>[2x]ADPGTSECSVIGYNAICINRGLHQVPELPAHVNYVDLSLNSIAELNETSFSRLQDLQFLKVEQQTPGLVIRNNTFRGLSSLIILKLDYNQFLQLETGAFNGLANLEVLTLTQCNLDGAVLSGNFFKPLTSLEMLVLRDNNIKKIQPASFFLNMRRFHVLDLTFNKVKSICEEDLLNFQGKHFTLLRLSSITLQDMNEYWLGWEKCGNPFKNTSITTLDLSGNGFKESMAKRFFDAIAGTKIQSLILSNSYNMGSSFGHTNFKDPDNFTFKGLEASGVKTCDLSKSKIFALLKSVFSHFTDLEQLTLAQNEINKIDDNAFWGLTHLLKLNLSQNFLGSIDSRMFENLDKLEVLDLSYNHIRALGDQSFLGLPNLKELALDTNQLKSVPDGIFDRLTSLQKIWLHTNPWDCSCPRIDYLSRWLNKNSQKEQGSAKCSGSGKPVRSIICPTSASLVPR;>GSAKDPGQIRGLEMASKNSQDGISLIQTAEGALTETHAILQRMRELTVQAGNTGTQQAEDLGAIKDEMDALIEEIDGISNRTEFNGKKLLDGTNSTDGFTFQIGANAGQQLNVKIDSMSSTALGVNALDVTDFAATAFDDQLKSIDTAINTVSTQRAKLGAVQNRLEHTINNLGASGENLTAA[2x]

Flagellin is a structural protein that assembles into the lash-like filament of a bacterial flagellum, which extends from the cell surface and allows bacteria to be motile. Upon bacterial invasion, flagellin is detected by Toll-like receptor 5 (TLR5) and NAIP5/NLRC4 in the host and activates innate immunity, contributing to the immediate clearance of pathogens from the host. TLR5 is an innate immune receptor located on the cell surface, and consists of an extracellular leucine-rich repeat (LRR) domain, a transmembrane domain, and an intracellular domain7. TLR5 recognizes flagellin as a pathogen-associated molecular pattern using the extracellular domain and activates the MyD88-dependent signaling pathway and NF-κB-mediated production of proinflammatory cytokines.

To reveal the structural mechanism of TLR5 binding to Gram-positive bacterial flagellin that lacks the hypervariable domains, the crystal structure of rTLR5N14 in complex with the central region of bsflagellin (bsflagellincent; D1 residues 54–230) was determined at 2.1 Å resolution. Consistent with the biophysical assays performed in solution, bsflagellincent formed a 1:1 complex with rTLR5N14 in the crystal structure. bsflagellincent forms a 1:1 complex with rTLR5N14 using a primary binding interface created between three long α-helices (αD1a, αD1b, and αD1c) of the bsflagellin D1 domain and the concave and lateral sides of TLR5. Although bsflagellin lacks the hypervariable domains, the bsflagellincent-rTLR5N14 complex adopts a similar 1:1 architecture as the sdflagellinD1-D2-rTLR5N14 complex. In the bsflagellincent-rTLR5N14 structure, the primary binding interface is divided into two regions, interface-A and interface-B, which are located at LRRNT-LRR6 and LRR7-LRR10 and have buried surface areas of 550 Å2 and 695 Å2, respectively. A comparative structural analysis of the bsflagellincent-rTLR5N14 and sdflagellinD1-D2-rTLR5N14 complexes suggests that the LRR9 loop of TLR5 centered in interface-B plays a critical role in both bsflagellin and sdflagellin binding. In the bsflagellincent-rTLR5N14 structure, bsflagellin R89 protrudes and is snugly inserted into a cavity that is generated by TLR5 LRR9 loop residues (Y267, N268, G270, S271, S272, H275, N277, F278, and K303). The side chain of bsflagellin R89 is enclosed by the side chains of TLR5 Y267, N268, S272, F278, and K303, that form the cavity wall, through van der Waals interactions and is stably hydrogen-bonded to the main-chain oxygen atoms of TLR5 cavity residues (Y267, G270, and S271). Thus, the R89A mutation in bsflagellin ablates the shape and chemical complementarity between bsflagellin R89 and the TLR5 LRR9 loop.> ASSLPPNALKPAFGPPDKVAAQKFKESLMATEKHAKDTSNMWVKISVWVALPAIALTAVNTYF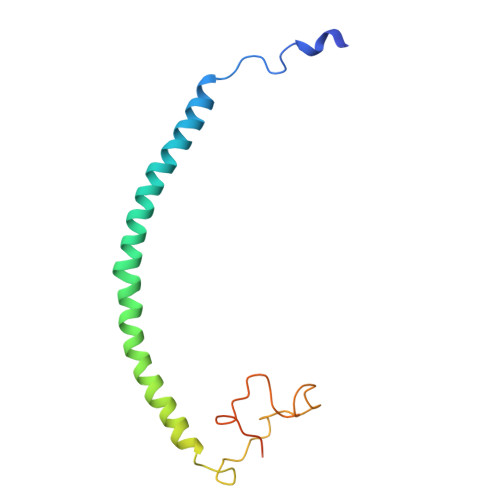VEKEHAEHREHLKHVPDSEWPRDYEFMNIRSKPFFWGDGDKTLFWNPVVNRHIEHDDGARGSHHHHHH>HHHHHIEGRHMAGPDRAELAELVRRLSVVHGRVTLSSGREADYYVDLRRATLHHRASALIGRLMRELTADWDYSVVGGLTLGADPVATAIMHAPGRPIDAFVVRKSAKAHGMQRLIEGSEVTGQRVLVVEDTSTTGNSALTAVHAVQDVG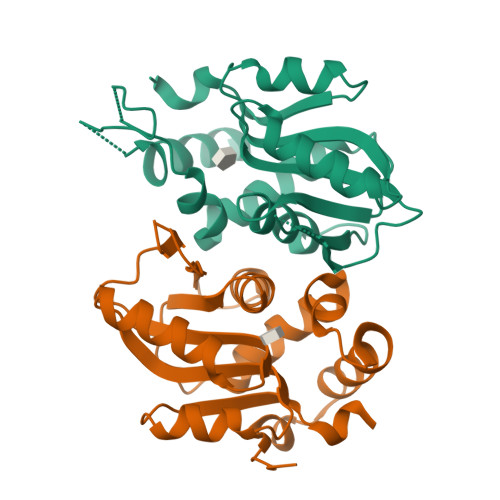GEVVGVATVVDRATGAAEAIEAEGLRYRSVLGLADLGLD[2x]> SNAMTIKGRAFPEGFLWGGAVAAHQLEGGYKEGGKGLSTADIMTLGTNERPREITDGVVAGKYYPNHQAIDFYHRYPEDIELFAEMGFKCFRTSIAWTRIFPNG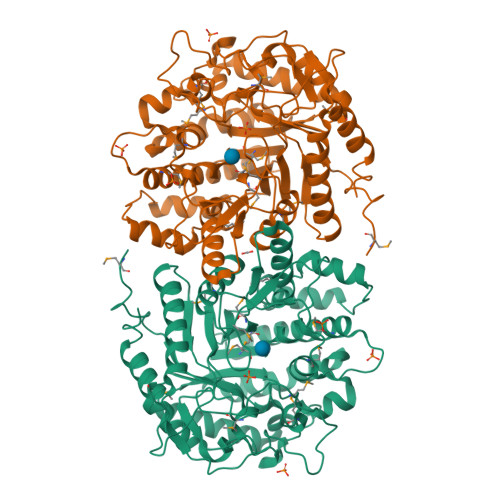DESEPNEAGLQFYDDLFDECLKNGIQPVVTLAHFEMPYHLVKQYGGWRNRKLIQFYLNFAKVCFERYRDKVTYWMTFNEINNQTNFESDGAMLTDSGIIHQPGENRERWMYQAAHYELVASAAAVQLGHQINPDFQIGCMIAMCPIYPLTAAPADVLFAQRAMQTRFYFADVHCNGTYPQWLRNRFESEHFNLDITAEDLKILQAGTVDYIGFSYYMSFTVKDTGKLAYNEEHDLVKNPYVKASDWGWQVDPVGLRYAMNWFTDRYHLPLFIVENGLGAIDKKTADNQIHDDYRIDYLTDHLRQIKLAVLEDGVDLIGYTPWGCIDLVAASTGQMSKRYGFIYVDENDDGSGSLKRYKKDSFTWFQHVIATNGAEIE>[2x]MRPLVATVDLSAIRHNYALAKRCAPQRQAFAVVKANA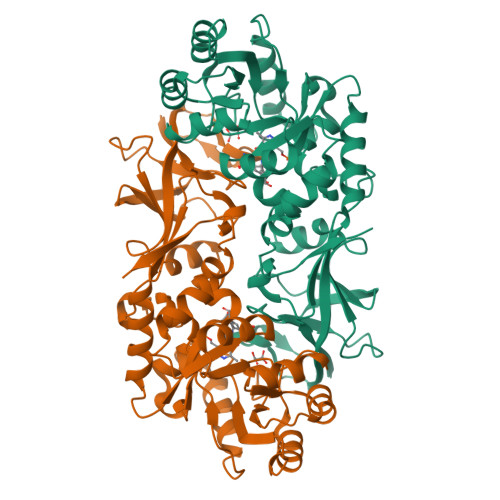YGHGAREVVTALHDDADGFAVACLEEAAEVRALHASARILLLEGCFEASEYALAGQLRLDLVIQGAEQGEAFLAAGLDIPLNVWLKLDSGMHRLGFDPAALRAWHARLRSHPGVRELNLISHFACADERNHPLTEQQLESFLGLLDLDFDQRSLANSAAVLTIPAAHMDWLRPGIMLYGSTPLADLSAAELGLKPAMSLGAQLISLREVAVGESVGYGATWIAERPARIGTVSCGYADGYPRTAPAGTPVLVGGRRAILAGRVSMDMLAVDLSDLPEARVGDPVELWGAGLSVDEVARACGTLGYELLSKVTARVPRRYSH3-[(4-fluorophenyl)sulfanyl]-N-(4-methyl-1,3-thiazol-2-yl)-6-[(4-methyl-4H-1,2,4-triazol-3-yl)sulfanyl]pyridine-2-carboxamide 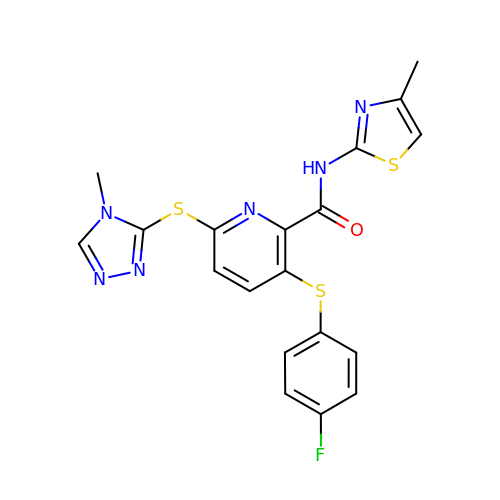| C19 H15 F N6 O S3 | SJTQKYKXCYVFHX-UHFFFAOYSA-N> ARTK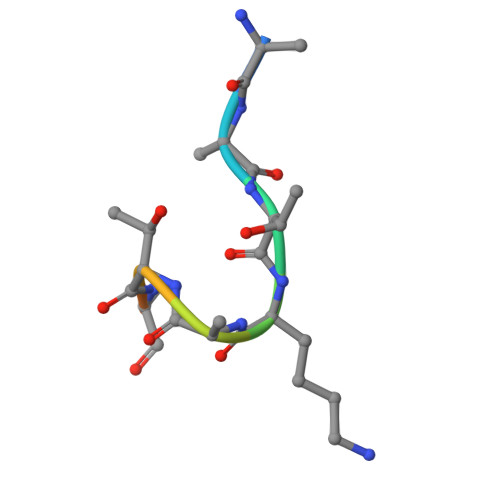QTARKS>[2x]GMFDYSAHPELLKGRVILVTGAARGIGAAAARAYAAHGASVVLLGRTEASLAEVSDQIKSAGQPQPLIIALNLENATAQ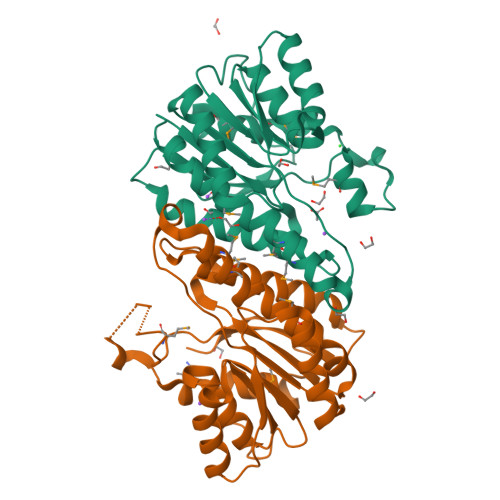QYRELAARVEHEFGRLDGLLHNASIIGPRTPLEQLPDEDFMQVMHVNVNATFMLTRALLPLLKRSEDASIAFTSSSVGRKGRANWGAYGVSKFATEGLMQTLADELEGVTAVRANSINPGATRTGMRAQAYPDENPLNNPAPEDIMPVYLYLMGPDSTGINGQALNAQ> TTVYLAGDSTMAKNGGGSGTNGWGEYLASYLSATVVNDAVAGRSARSYTREGRFENIADVVTAGDYVIVEFGHNDGGSLSTDNGRTDCSGTGAEVCYSVYDGVNETILTFPAYLENAAK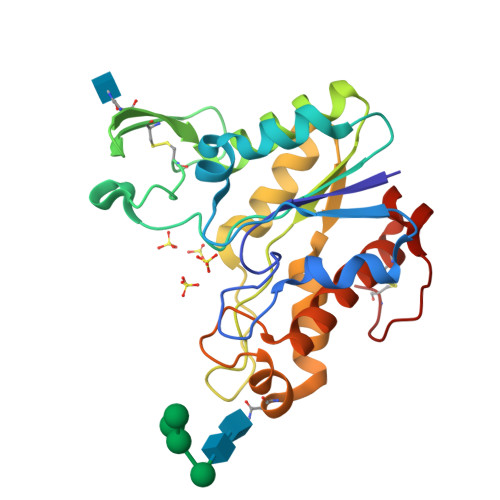LFTAKGAKVILSSQTPNNPWETGTFVNSPTRFVEYAELAAEVAGVEYVDHWSYVDSIYETLGNATVNSYFPIDHTHTSPAGAEVVAEAFLKAVVCTGTSLKSVLTTTSFEGTCL>[2x]M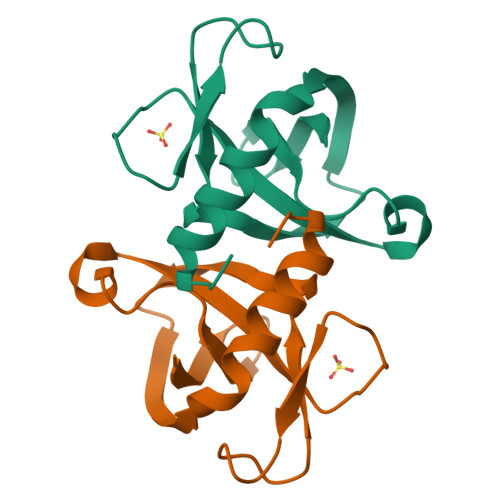RPIHIAQLDKARPVLILTREVVRPHLTNVTVAPITTTVRGLATEVPVDAVNGLNQPSVVSCDNTQTIPVCDLGRQIGYLLASQEPALAEAIGNAFDLDWVVA> MKLSKDTIAILKNFASINSGILLSQGKFIMTRAVNGTTYAEANISDEIDFDVALYDLNSFLSILSLVSDDAEISMHTDGNIKIADTRSTVYWPAADKS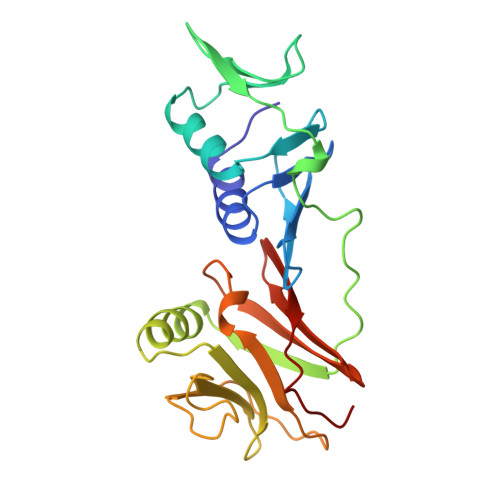TIVFPNKPIQFPVASVITEIKAEDLQQLLRVSRGLQIDTIAITNKDGKIVINGYNKVEDSGLTRPKYSLTLTDYDGSNNFNFVINMANMKIQPGNYKVMLWGAGDKVAAKFESSQVSYVIAMEADSTHDF methyl 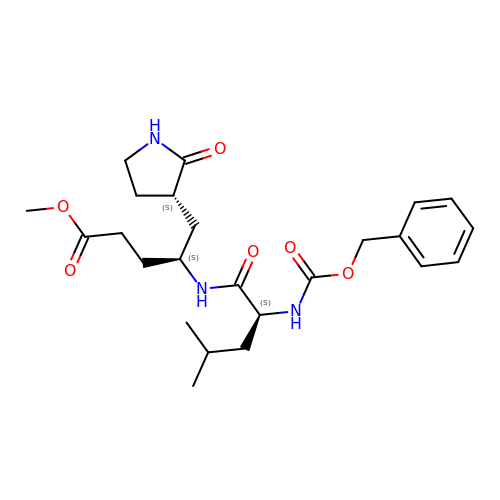(4~{S})-4-[[(2~{S})-4-methyl-2-(phenylmethoxycarbonylamino)pentanoyl]amino]-5-[(3~{S})-2-oxidanylidenepyrrolidin-3-yl]pentanoate | C24 H35 N3 O6 | JGJNNQJIGUGNAT-UFYCRDLUSA-N To extend the structural coverage of proteins of unknown function, we targeted Pfam protein family PF06684 (domain of unknown function 1185; DUF1185) and determined the crystal structures of two representative members. Despite lacking any recognizable sequence similarity to other protein families, both proteins show significant structural similarity to proteins with a Bacillus chorismate mutase-like (BCM-like) fold characterized by a β-α-β-α-β-β core that includes a mixed β-sheet (order 1423) with the β4 strand antiparallel to the rest. The biological unit of both proteins is a hexamer and analysis of homologs indicates that the oligomer interface residues are highly conserved. Structural similarities to BCM and genome-context analysis suggest a function in amino-acid synthesis.

The SPO0826 gene of the marine α-proteobacterium Silicibacter pomeroyi encodes a protein with a molecular weight of 20.5 kDa (residues 1–­193) and a calculated isoelectric point of 6.2. The crystal structure of SPO0826 was determined to 2.1 Å resolution using the MAD method. The final model included one protomer (147 of 194 residues) and 42 water molecules in the asymmetric unit. No electron density was observed for residues from the expression and purification tag, SeMet1–Thr2, Gly103–Ala115, Lys137–His145 or Gly172–Arg193. SPO0826 also forms a single domain composed of seven β-strands (β1–β7; residues 4–17, 20–36, 78–85, 119–123, 130–134, 147–151 and 161–170), but with only two α-helices (H1 and H3; residues 48–69 and 91–97) and one 310-helix (H2; residues 73–75). The dis­ordered residues in the SPO0826 structure correspond to a large C-­terminal region of BB2672 that encompasses helix H4 (residues 97–109), most of the H4–β4 loop (residues 110–115), the β5–β6 loop (residues 137–145), including the 310-helix H5, and the C-terminal region (residues 172–193) after β7, including 310-helix H6. However, this interface was not observed in the SPO0826 structure, which crystallized with a single molecule in the asymmetric unit. In BB2672, the N-terminal interface is involved in the formation of the hexamer, while in SPO0826, it is only involved in crystal contacts. The observation that SPO0826 crystallizes as a monomer in high salt and acidic pH (2 M NaCl pH 6.5), while demonstrating the same hexameric oligomerization state in solution as BB2672 under alkaline and low-salt conditions (150 mM NaCl pH 8.0), lends further support to the hypothesis that pH or salt concentration might be a key factor in oligomerization.

> GMTKIRKIAVFIEETRIEAGREISPPTRKAVAVAVIENPFAGRYVEDLTELMDTGAELGALLGERCVQALGIRPEQAESYGKSAMVGENGELEHAAAILHPKLGAPLRKAVEKGAALVPSSKKMGSPGQVLDVPLGHKDAAYVRSHFDGIEVRLNDAPRANEIMVAVAVTDSGRPLPRVGGLTHDAAEGKDGLR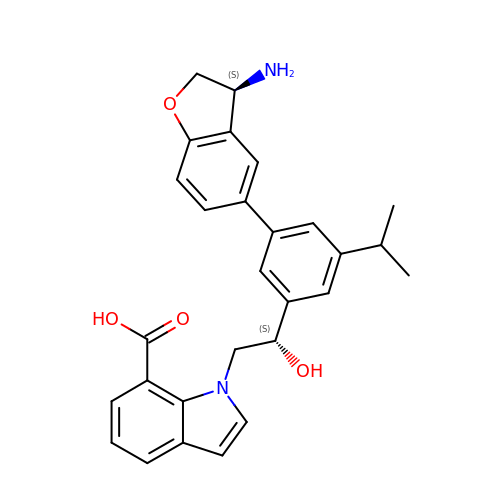1-[(2S)-2-{3-[(3S)-3-amino-2,3-dihydro-1-benzofuran-5-yl]-5-(propan-2-yl)phenyl}-2-hydroxyethyl]-1H-indole-7-carboxylic acid | C28 H28 N2 O4 | GOERAAJVARXHDP-JWQCQUIFSA-N>[5x]MRRAVGVPPVMAYAEGPPPSYESVMGSADSPATLEALYVPPRYLGPTEGRNSIRYSELAPLYDTTRVYLVDNKSADIASLNYQNDHSNFQTTVVQNNDFTPAEAGTQTINFDERSRWGADLKTILRTNMPNINEFMST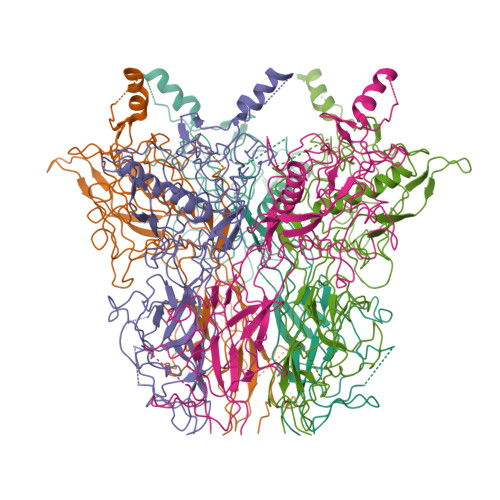NKFKARLMVEKKNKETGLPRYEWFEFTLPEGNYSETMTIDLMNNAIVDNYLEVGRQNGVLESDIGVKFDTRNFRLGWDPVTKLVMPGVYTNEAFHPDIVLLPGCGVDFTQSRLSNLLGIRKRLPFQEGFQIMYEDLEGGNIPALLDVAKYEASIQKAKEEGKEIGDDTFATRPQDLVIEPVAKDSKNRSYNLLPNDQNNTAYRSWFLAYNYGDPKKGVQSWTLLTTADVTCGSQQVYWSLPDMMQDPVTFRPSTQVSNYPVVGVELLPVHAKSFYNEQAVYSQLIRQSTALTHVFNRFPENQILVRPPAPTITTVSENVPALTDHGTLPLRSSISGVQRVTITDARRRTCPYVHKALGIVAPKVLSSRTF> GSSALLDTDEVGSELD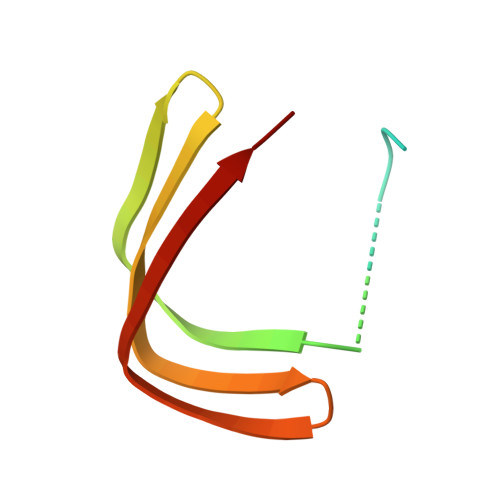DSDDDYLISEGEEDGPDENLMLCLYDKVTRTKARWKCSLKDGVVTINRNDYTFQKAQVEAEWV>[4x]SAPRPCQAPQQWEGRQVMYQ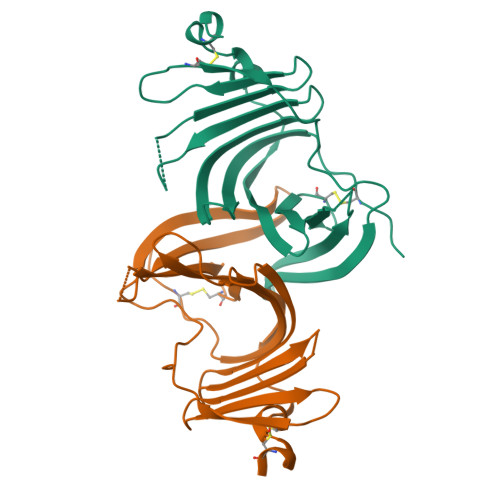QSSGRNSRALLSYDGLNQRVRVLDERKALIPCKRLFEYILLYKDGVMFQIDQATKQCSKMTLTQPWDPLDIPQNSTFEDQYSIGGPQEQITVQEWSDRKSARSYETWIGIYTVKDCYPVQETFTINYSVILSTRFFDIQLGIKDPSVFTPPSTCQMAQLEKMSEDCSWHHHHHH> MSAKNNTHHFPKLLILVGAPGSGKSTFARYFIRTEDNWVRVNRDDFRLMQFGDSLMSPFYEERITKMVEASVIALLKNRTNVIIDATNSSLRSLQDMVHTYTEYADISFKVFDLPVEELVKRCDKRCEQTGKFIPKSAIEKHVTQLQYTKEKFDFKPIPRALKETSLTYADQDTSLP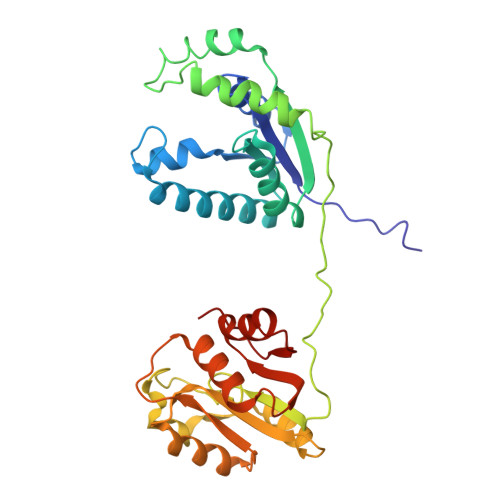KAVICDLDGTLSLLNGRDPYNASTADQDLLNTPVAMVLKMAKQQGYKVILLSGRENAYREPTERFLAKYQIDYDLLLMRDTNDYRKDNIIKKELFLEEIQGKYFVEFLLDDRNQVVDMWRRELALPCFQVNYGDF> MKRDHHQFQGRLSNHGTSSSSSSISKDKMMMVKKEEDGGGNMDDELLAVLGYKVRSSEMAEVALKLEQLETMMSNVQEDGLSHLATDTVHYNPSELYSWLDNMLSELNPPPLPASSNGLDPVLPSPEICGFPASDYDLKVIPGNAIYQFPAIDSSSSSNNQNQQLQSCSSPDSMVTSTSTGTQIGGVIGTTVTTTTTTTTAAGESTRSVILVDSQENGVRLVHALMACAEAIQQNNLTLAEALVKQIGCLAVSQAGAMRKVATYFAEALARRIYRLSPPQNQIDHCLSDTLQMHFYETCPYLKFAHFTANQAILEAFEGKKRVHVIDFSMNQGLQWPALMQALALREGGPPTFRLTGIGPPAPDNSDHLHEVGCKLA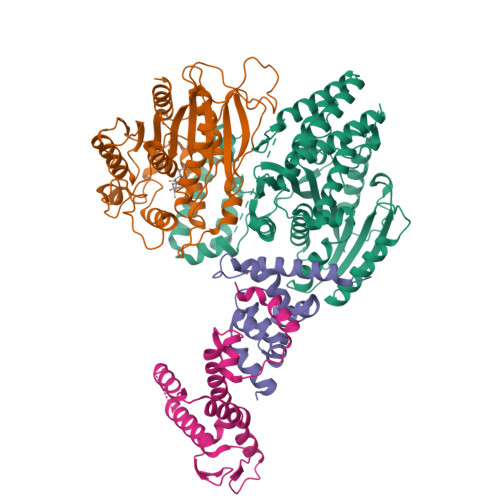QLAEAIHVEFEYRGFVANSLADLDASMLELRPSDTEAVAVNSVFELHKLLGRPGGIEKVLGVVKQIKPVIFTVVEQESNHNGPVFLDRFTESLHYYSTLFDSLEGVPNSQDKVMSEVYLGKQICNLVACEGPDRVERHETLSQWGNRFGSSGLAPAHLGSNAFKQASMLLSVFNSGQGYRVEESNGCLMLGWHTRPLITTSAWKLSTAAYGGWSHPQFER;> MAASDEVNLIESRTVVPLNTWVLISNFKVAYNILRRPDGTFNRHLAEYLDRKVTANANPVDGVFSFDVLIDRRINLLSRVYRPAYADQEQPPSILDLEKPVDGDIVPVILFFHGGSFAHSSANSAIYDTLCRRLVGLCKCVVVSVNYRRAPENPYPCAYDDGWIALNWVNSRSWLKSKKDSKVHIFLAGDSSGGNIAHNVALRAGESGIDVLGNILLNPMFGGNERTESEKSLDGKYFVTVRDRDWYWKAFLPEGEDREHPACNPFSPRGKSLEGVSFPKSLVVVAGLDLIRDWQLAYAEGLKKAGQEVKLMHLEKATVGFYLLPNNNHFHNVMDEISAFVNAECGGDYKDDDDK;> HHHHHHHHHHENLYFQSHMKRSTTDSDLAGDAHNETNKKMKSTEEEEIGFSNLDENLVYEVLKHVDAKTLAMSSCVSKIWHKTAQDERLWELICTRHWTNIGCGQNQLRSVVLALGGFRRLHSLYLWPLSKPNPRARFGKDELKLTLSLLSIRYYKKMSFTKRPLPESKGGWSHPQFER;> HHHHHHHHHHENLYFQSHMSAKKIVLKSSDGESFEVEEAVALESQTIAHMVEDDCVDNGVPLPNVTSKILAKVIEYCKRHVEAAASKAEAVEGAATSDDDLKAWDADFMKIDQATLFELILAANYLNIKNLLDLTCQTVADMIKGKTPEEIRTTFNIKNDFTPEEEEEVRRENQWAFEGGYKDDDDK O-ACETALDEHYDYL-HEXAETHYLENE 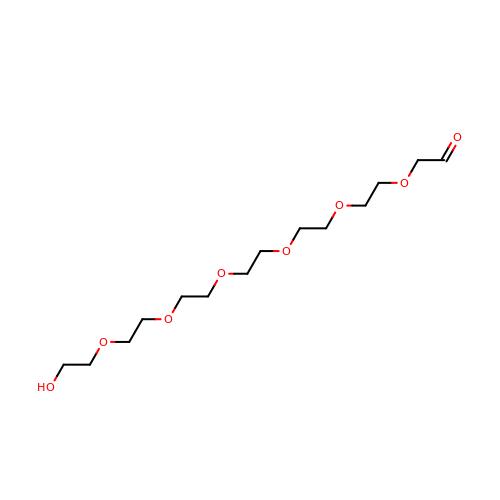GLYCOL | C14 H28 O8 | CTLLATPOKUEFSQ-UHFFFAOYSA-N> GSHMEKLAKNKVISIDAGRKY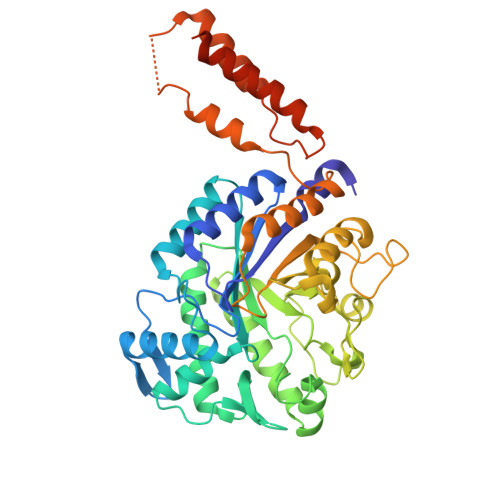FTLNQLKRIVDKASELGYSDVHLLLGNDGLRFLLDDMTITANGKTYASDDVKKAIIEGTKAYYDDPNGTALTQAEVTELIEYAKSKDIGLIPAINSPGHMDAMLVAMEKLGIKNPQAHFDKVSKTTMDLKNEEAMNFVKALIGKYMDFFAGKTKIFNFGTDEYANDATSAQGWYYLKWYQLYGKFAEYANTLAAMAKERGLQPMAFNDGFYYEDKDDVQFDKDVLISYWSKGWWGYNLASPQYLASKGYKFLNTNGDWYYILGQKPEDGGGFLKKAIENTGKTPFNQLASTKYPEVDLPTVGSMLSIWADRPSAEYKEEEIFELMTAFADHNKDYFRANYNALREELAKIPTNLEGYSKESLEALDAAKTALNYNLNRNKQAELDTLVANLKAALQGKKPAVTHSGSLDENEVAANVETRP>[10x]MRSFLNLNSIPNVAAGNSCSIKLPIGQTYEVIDLRYSGVTPSQIKNVRVELDGRLLSTYKTLNDLILENTRHKRKIKAGVVSFHFVRPEMKGVNVTDLVQQRMFALGTVGLTTCEIKFDIDEAAAGPKLSAIAQKSVGTAPSWLTMRRNFFKQLNNGTTEIADLPRPVGYRIAAIHIK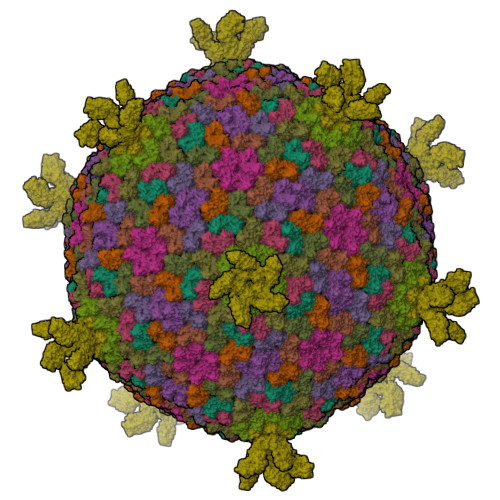AAGVDAVEFQIDGTKWRDLLKKADNDYILEQYGKAVLDNTYTIDFMLEGDVYQSVLLDQMIQDLRLKIDSTMDEQAEIIVEYMGVWSRNGF;> MIVKKKLAAGEFAETFKNGNNITIIKAVGELVLRAYGADGGEGLRTIVRQGVSIKGMNYTSVMLHTEYAQEIEYWVGDLDYSFQEQTTKSRDVNSFQIPLRDGVRELLPEDASRNRASIKSPVDIWIGGENMTALNGIVDGGRKFEAGQEFQINTFGSVNYWVSDEEIRVFKEYSARAKYAQNEGRTALEANNVPFFDIDVPPELDGVPFSLKARVRHKSKGVDGLGDYTSISVKPAFYITEGDETTDTLIKYTSYGSTGSHSGYDFDDNTLDVMVTLSAGVHRVFPVETELDYDAVQEVQHDWYDESFTTFIEVYSDDPLLTVKGYAQILMERT;>MNTSVPTSVPTNQSVWGNVSTGLDALISGWARVEQIKAAKASTGQGRVEQAMTPELDNGAAVVVEAPKKAAQPSETLVFGVPQKTLLLGFGGLLVLGLVMRGNK[4x];> MANFLTKNFVWILAAGVGVWFYQKADNAAKTATKPIADFLAELQFLVNGSNYVKFPNAGFVLTRDALQDDFIAYDDRIKAWLGTHDRHKDFLAEILDHERRVKPVYRKLIGNIIDASTIRAASGVEL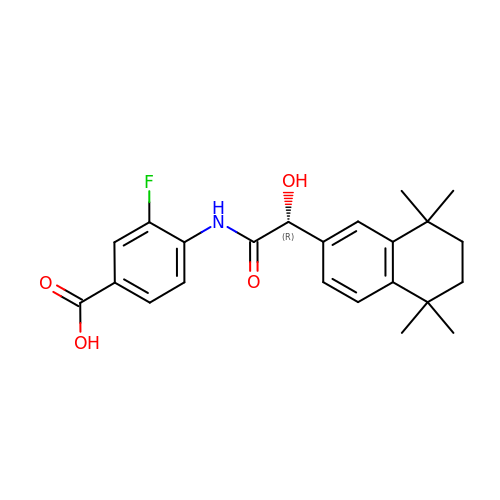R-3-FLUORO-4-[2-HYDROXY-2-(5,5,8,8-TETRAMETHYL-5,6,7,8,-TETRAHYDRO-NAPHTALEN-2-YL)-ACETYLAMINO]-BENZOIC ACID | C23 H26 F N O4 | AANFHDFOMFRLLR-LJQANCHMSA-N> EELQKSIGHKPEPTDEEWELIKTVTEAHVATNAQGSHWKQKRKFLPEDIGQAPIVNAPEGG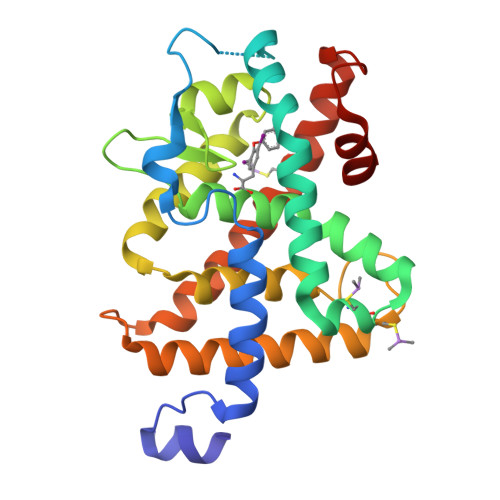KVDLEAFSHFTKIITPAITRVVDFAKKLPMFCELPCEDQIILLKGCCMEIMSLRAAVRYDPESETLTLNGEMAVTRGQLKNGGLGVVSDAIFDLGMSLSSFNLDDTEVALLQAVLLMSSDRPGLACVERIEKYQDSFLLAFEHYINYRKHHVTHFWPKLLMKVTDLRMIGACHASRFLHMKVECPTELFPPLFLEVFE>GPGRAKIDVDSVDHTDDYIHLRKWIKRIGIILRISGHWPFRLPHEKRNQHKSKFRQVYSCLVITLGFITCSCYCIGLCLSESIAQALNNITVTSYFLQSCVCYVSFIINSRKLETLFNYLFENEVVGCPRGYKMSSIKTTLFRCKFVAFSLGILSFFGWLMWTLLPLAVLVVDSGATGGGNQTSLRFVEAWYPFDTTTSPMNEVIAIYEAVAMIFLITAPMSSDIMFCVLMIFIVEHLKCLGMAIECTLKGISTNQHQNIGFDDSVSDVNVQRRIVIGKESPIQSIHVPIKECSRQSSDAVFREKRHGTHHQIIRSHNYTDATSLCNIVDSHVKIYRTMEIVQSVYSSYFATLFFTSCLAVCALAYFLAATSTSFTRVPGMVLYLMYIFLRIFLLCLLATEVAEQGLNLCHAGYSSKLVLASDHVRSTIQAIATRAQIPLSITGARFFTV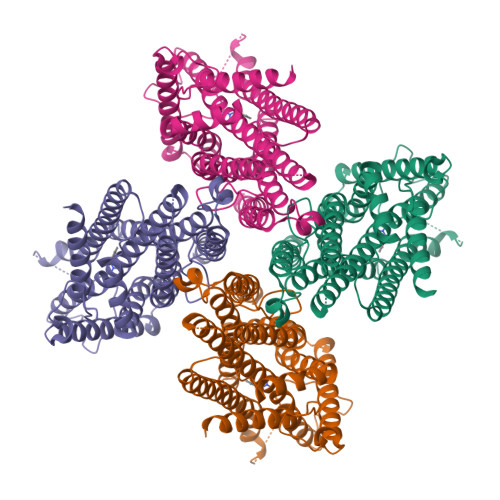NLSFLASMAGVMLTYFIVLLQVNAKPKP[4x]>[8x]TVEPVL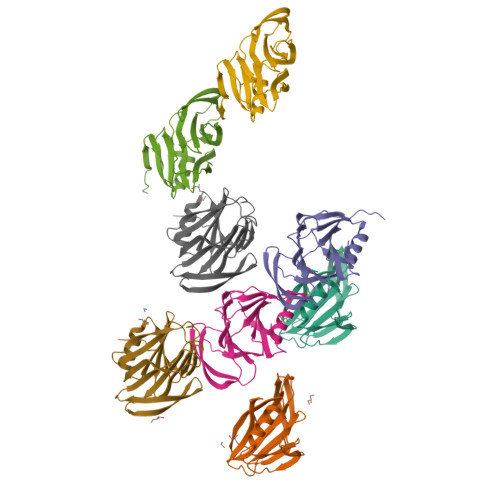DGPYQPTTFKPPNDYWLLISSNTNGVVYESTNNNDFWTAVIAVEPHVSQTNRQYILFGENKQFNVENNSDKWKFFEMFKGSSQGDFSNRRTLTSSNRLVGMLKYGGRVWTFHGETPRATTDSSNTADLNNISIIIHSEFYIIPRSQESKCNEYINNGL> MAVTNEEIKTASKIVRRVSNVEAFDKSGSVFKGYQIWTDISPTIENDPNIMFVKCVVQQGSKKEKLTVVQIDPPGTGTPYDIDPTHAWNCNSQVDPMSFGDIGLLNHTNIPCVLDFLKHRYLKNQIYTTAVPLIVAINPYKDLGNTTNEWIRRYRDTADHTKLPPHVFTCAREALSNLHGVNKSQTIIVSGESGAGKTEATKQIMRYFASSKSGNMDLRIQTAIMAANPVLEAFGNAKTIRNNNSSRFGRFMQLVISHEGGIRYGSVVAFLLEKSRIITQDDNERSYHIFYQFLKGANSTMKSKFGLKGVTEYKLLNPNSTEVSGVDDVKDFEEVIESLKNMELSESDIEVIFSIVAGILTLGNVRLIEKQEAGLSDAAAIMDEDMGVFNKACELMYLDPELIKREILIKVTVAGGTKIEGRWNKNDAEVLKSSLCKAMYEKLFLWIIRHLNSRIEPEGGFKTFMGMLDIFGFEVFKNNSLEQLFINITNEMLQKNFVDIVFERESKLYKDEGISTAELKYTSNKEVINVLCEKGKSVLSYLEDQCLAPGGTDEKFVSSCATNLKENNKFTPAKVASNKNFIIQHTIGPIQYCAESFLLKNKDVLRGDLVEVIKDSPNPIVQQLFEGQVIEKGKIAKGSLIGSQFLNQLTSLMNLINSTEPHFIRCIKPNENKKPLEWCEPKILIQLHALSILEALVLRQLGYSYRRTFEEFLYQYKFVDIAAAEDSSVENQNKCVNILKLSGLSESMYKIGKSMVFLKQEGAKILTKIQREKLVEWENCVSVIEAAILKHKYKQKVNKNIPSLLRVQAHIRKKMVAQ;> MKQECNVCYFNLPDPESTLGPYDNELNYFTWGPGFEYEPEPQRKPLSIEESFENSEESEESVADIQQLEEKVDESDVRIYFNEKSSGGKISIDNASYNARKLGLAPSSIDEKKIKELYGDNLTYEQYLEYLSICVHDKDNVEELIKMFAHFDNNCTGYLTKSQMKNILTTWGDALTDQEAIDALNAFSSEDNIDYKLFCEDILQ;> MASDMEEKFREAFILFSSCSDHIEMYKFFELMNSFGIILTNDEKAALPNDINMDYWLNFAKKHYNYEQPFKHINNVNEQNTNVQIKIDNFLGIMKALDTRLTESDLNILLQITNPENKST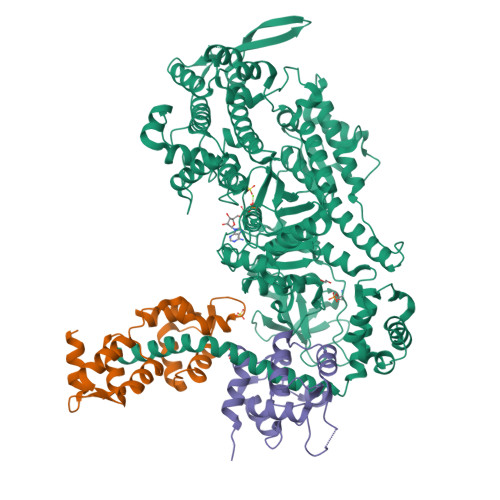LNLKTVSQKLTESI4-(2-HYDROXYPHENYLTHIO)-1-BUTENYLPHOSPHONIC ACID 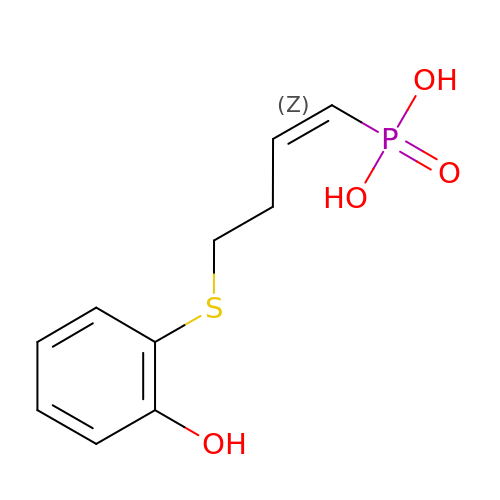| C10 H13 O4 P S | GHNIEXOPSISMGX-XVNBXDOJSA-N> VTDSINWASGEDDHVVARAEYDFAAVSEEEISFRAGDMLNLALKEQQPKVRGWLLASLDGQTTGLIPANYVKILGKRKGRKTVESS

Import of proteins into peroxisomes depends on PEX5, PEX13 and PEX14. By combining biochemical methods and structural biology, we show that the C-terminal SH3 domain of PEX13 mediates intramolecular interactions with a proximal FxxxF motif. The SH3 domain also binds WxxxF peptide motifs in the import receptor PEX5, demonstrating evolutionary conservation of such interactions from yeast to human. Strikingly, intramolecular interaction of the PEX13 FxxxF motif regulates binding of PEX5 WxxxF/Y motifs to the PEX13 SH3 domain.

Structures of the apo SH3 domain and SH3-(GS)2-FxxxF were solved by X-ray crystallography at 1.8Å and 2.3Å resolution, respectively. Analysis of the structure of the SH3 domain shows a network of polar contacts between the N- and C-terminal regions stabilizing the β1/β5 interaction, consistent with the extended domain boundaries observed by NMR. NMR {1H}-15N heteronuclear NOE (hetNOE) data, which report on backbone dynamics at sub nanosecond timescales, indicate that the PEX13 SH3 fold extends beyond the typical SH3 structural elements compared to the yeast Pex13 and other human SH3 domains. A comparison of the apo PEX13 SH3 and the complex structure show that the SH3 fold is highly similar (backbone coordinate RMSD = 0.39). Interestingly, nine out of the eleven Arg and Lys residues are located at the FxxxF binding surface, forming a positively charged surface area, which is favorable for binding negatively charged peptides such as the C-terminal FxxxF motif. In contrast, the PxxP binding site located at the opposite side of the SH3 domain, is mostly negatively charged. Notably, the human PEX13 SH3 interacts with (di)aromatic peptide motifs on a surface opposite to the PxxP binding region, as has previously been reported for yeast Pex1326.Substrate-binding proteins (SBPs) are key structural elements of the ABC transporter system that determine the substrate specificity and high affinity of the ABC uptake system. A typical SBP consists of two α/β domains, which are connected by a hinge region. To understand their molecular functions, we performed a crystallographic study of single domain SBP from Rhodothermus marinus (RmSBP). The overall structure of RmSBP showed the single α/β fold, which is identical with that previous reported, although the molecular flexibility was distinct.

The crystal of RmSBP soaked with NaBr (RmSBP-Br) belongs to the orthorhombic P212121 space group with unit cell parameters a = 92.84, b = 97.86, and c = 101.98 Å, containing one RmSBP molecule per asymmetric unit. The crystal structure of RmSBP-Br showed the three disordered regions at the α2-helix (Arg58–Gln64), the loop between β5-and β6-strands (Asp151–Gly154), and the C-terminus (Gln176–Leu182). These three disordered regions were shown to have relative flexibility in the previous crystal structure analysis, but were clearly disordered in RmSBP-Br. Although NaBr was used for soaking, no electron density map corresponding to a Br ion was observed, and it is possible that NaBr had diffused in the solvent regions in crystal packing, increasing the flexibility of the three disordered regions. This indicates that these regions of RmSBP are likely to be dynamic in a tentatively solution state. However, the position of three disordered regions of RmSBP was not directly related to the previously predicted substrate-binding site of RmSBP. Therefore, these regions may be involved in interactions with potential partner molecules or receptor proteins. The sequences of the disordered α2-helix (Arg58–Gln64), loop between the β5-and β6-strands (Asp151–Gly154), and C-terminus (Gln176–Leu182) in RmSBP-Br are similar to those of RpSBP and potentially have a similar molecular flexibility.

> MHTLRLFTVLSLLLTSAFTLFPETETEVTPIQQLFLIKELKPGIARIGVIWDKNAANRDEVLPQLQRASAATGIKVVVAEVASLQEVAPQFRTLLRDHQVEALWVLEESGLLGQAAARSFLIKNATQAGMPVFAPSETWLKEGACVTWRKDAEGIRLVVNKAVAEAMGITIPAKYQDRTAFLAMN> IEGYECQPIFLNVLEAIEPGVVCAGHDNNQPDSFAALLSSLNELGERQLVHVVKWAKALPGFRNLHVDDQMAVIQYSWMGLMVFAMGWRSFTNVNSRMLYFAPDLVF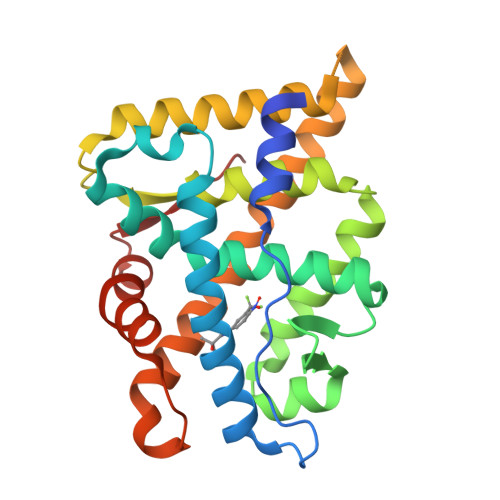NEYRMHKSRMYSQCVRMRHLSQEFGWLQITPQEFLCMKALLLFSIIPVDGLKNQKFFDELRMNYIKELDRIIACKRKNPTSCSRRFYQLTKLLDSVQPIARELHQFAFDLLIKSHMVSVDFPEMMAEIISVQVPKILSGKVKPIYFHTQ> REVLTGGHSVSAPQENRIYVMDSVFMHLTESRVHVYDYTNGKFLGMVPTAFNGHVQVSNDGKKIYTMTTYHERITRGKRSDVVEVWDADKLTFEKEISLPPKRVQGLNYDGLFRQTTDGKF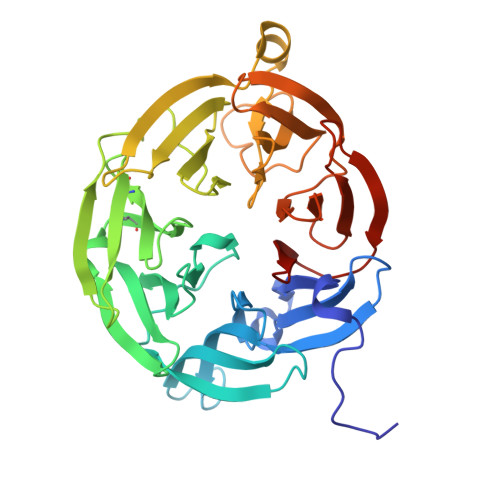IVLQNASPATSIGIVDVAKGDYVEDVTAAAGCWSVIPQPNRPRSFMTICGDGGLLTINLGEDGKVASQSRSKQMFSVKDDPIFIAPALDKDKAHFVSYYGNVYSADFSGDEVKVDGPWSLLNDEDKAKNWVPGGYNLVGLHRASGRMYVFMHPDGKEGTHKFPAAEIWVMDTKTKQRVARIPGRDALSMTIDQQRNLMLTLDGGNVNVYDISQPEPKLLRTIEGAAEASLQVQFHPVGGV As the most abundant viral protein encoded by the M gene segment, matrix protein 1 (M1) forms a shell underneath a host cell-derived lipid biolayer to connect the vRNPs with the viral envelope in mature virions. The full-length M1 protein includes 252 amino acids consisting of a highly organized N-terminal domain and a flexible but less ordered C-terminal domain that are linked by a protease-sensitive loop. So far, only the N-terminal domain of M1 has been structurally resolved at an atomic level, showing that at neutral pH the physiological monomers have a high tendency to oligomerize via a so-called ‘face-to-back’ arrangement, whereas at acidic pH the N-terminal domain exists as a dimeric structure in a so-called ‘face-to-face’ arrangement.

M(NLS-88R)-acidic has monomers A and B or C and D associated to form two independent physiological dimers (dimers 1 and 2, respectively) in the crystal. Least-squares superpositions of the four M(NLS-88R)-acidic monomers or superposition of its two independent dimers resulted in low r.m.s.d.s of 0.2–0.4 Å or 0.4 Å, suggesting similar quaternary conformation or monomer–monomer arrangements. Interactions between the monomers that form the face-to-face dimer in M(NLS-88R)-acidic, M(NLS-88E)-acidic or M(NLS-88E)-neutral involve hydrophobic contacts (mainly between the symmetry-related helices H6, and between helices H9 and loops L9), as well as several hydrogen-bond and/or salt-bridge interactions. When compared to the M(NLS-88E)-neutral dimer interface, the positively charged Lys104 side-chain in M(NLS-88R)-acidic has reoriented to avoid close contact with the positively charged opposing Arg88. In addition to these conserved inter-subunit hydrogen-bonds, the G88R mutation also results in an extra hydrogen-bond from Arg88-NE to Arg134-O in M(NLS-88)-acidic structure. This additional inter-subunit interaction may explain why it took longer for M(NLS-88R) M1 to disintegrate in vitro at pH 5.5 than wt-M1, as the fulcrum of M(NLS-88R)-acidic was relatively difficult to break during the dimer interface rotation. Of note, the face-to-face dimeric interaction is stronger than the face-to-back monomeric interaction as indicated by the BLI data. Thus, the acid-facilitated M1 conformational change is likely irreversible, presumably to prevent dissociated M1 from re-associating with vRNP in the cytosol after virus uncoating.

>MHHHHHHSLLTEVETYVLSIVPSGPLKAEIAQRLEDVFAGKNTDLEVLMEWLKTRPILSPLTKGILGFVFTLTVPSERGLQRRRFVQNALNGNRDPNNMDKAVKLYSKLKSEITFHGAKEIALSYSAGALASCMGLIYNRMGAVTTEVAFGLVCATCEQIADSQHRSHRQM[4x]> MAEPVSPLKHFVLAKKAITAIFDQLLEFVTEGSHFVEATYKNPELDRIATEDDLVEMQGYKDKLSIIGEVLSRRHMKVAFFGRTSSGKSSVINAMLWDKVLPSGIGHITNCFLSVEGTDGDKAY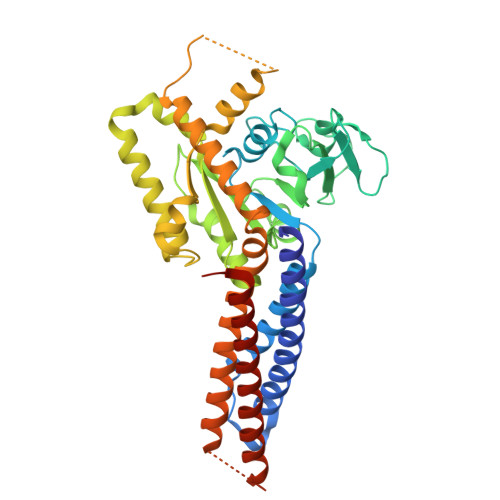LMTEGSDEKKSVKTVNQLAHALHMDKDLKAGCLVRVFWPKAKCALLRDDLVLVDSPGTDVTTELDSWIDKFCLDADVFVLVANSESTLMNTEKHFFHKVNERLSKPNIFILNNRWDASASEPEYMEDVRRQHMERCLHFLVEELKVVNALEAQNRIFFVSAKEVLSARKQKAQGMPESGVALAEGFHARLQEFQNFEQIFEECISQSAVKTKFEQHTIRAKQILATVKNIMDSVNLAAEDGSGSGSGGSEIARLPKEIDQLEKIQNNSKLLRNKAVQLENELENFTKQFLPSSNEES3-[(1R,2S,4R,6S)-2-ethenyl-4,6-dimethyl-cyclohexyl]-4-oxidanyl-1H-pyridin-2-one 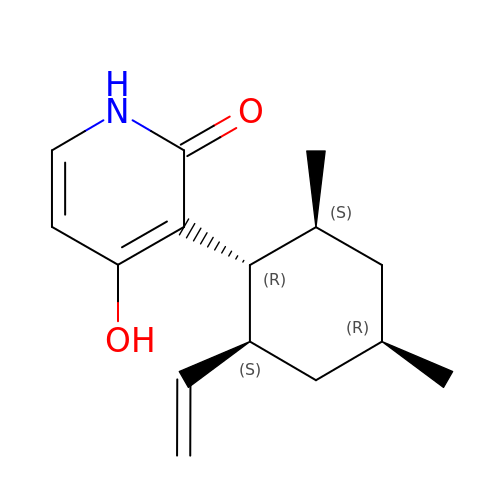| C15 H21 N O2 | SWIJWROLKBJDFO-LSCVPOLPSA-N>NSKDSIVNDDDDSTSEVDAIPDSTNPSGSFPSVEYDVFLSFRGPDTRKQFTDFLYHFLCYYKIHTFRDDDELRKGKEIGPNLLRAIDQSKIYVPIISSGYADSKWCLMELAEIVRRQEEDPRRIILPIFYMVDPSDVRHQTGCYKK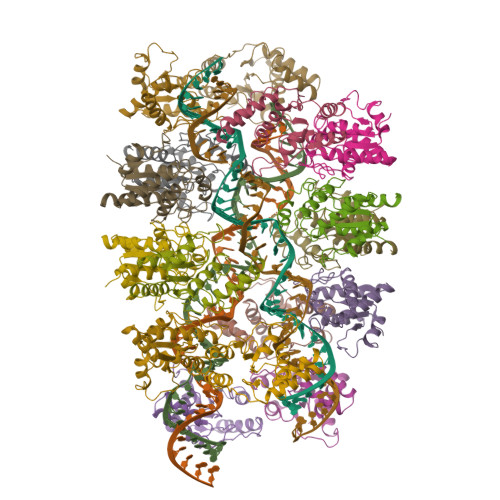AFRKHANKFDGQTIQNWKDALKKVGDLKGWHIGKDDEQGAIADKVSADIWSHISKENL[16x]>[2x]MKQYLELMQKVLDEGTQKNDRTGTGTLS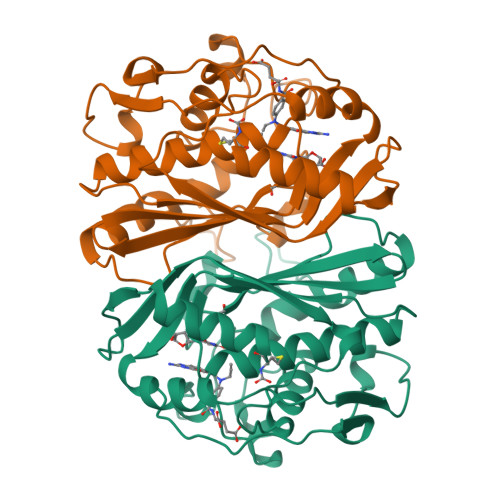IFGHQMRFNLQDGFPLVTTKRCHLRSIIHELLWFLQGDTNIAYLHENNVTIWDEWADENGDLGPVYGKQWRAWPTPDGRHIDQITTVLNQLKNDPDSRRIIVSAWNVGELDKMALAPCHAFFQFYVADGKLSCQLYQRSCDVFLGLPFAIASYALLVHMMAQQCDLEVGDFVWTGGDTHLYSNHMDQTHLQLSREPRPLPKLIIKRKPESIFDYRFEDFEIEGYDPHPGIKAPVAI> GSQPEQKTLSLPGTYRHVDRTTGQVLTCDKCPAGTYVSEHCTNMSLRVCSSCPAGTFTRHENGIERCHDCSQPCPWPMIERLPCAALTDRECICPPGMYQSNGTCAPHTVCPVGWGVRKKGTENEDVRCKQCARGTFSDVPSSVMKCKAHTDCLGQNLEVVKPGTKETDNVCGMRLFFSSTASGRGLVPR;> GSSTPDAVDKYLETPGDENEHAHFQKAKERLEAKHRERMSQVMREWEEAERQAKNLPKADKKAVIQHFQEKVESLEQEAANERQQLVETHMARVEAMLNDRRRLALENYITALQAVPPRPHHVFNMLKKYVRAEQKDRQHTLKHFEHVRMVDPKKAAQIRSQVMTHLRVIYERMNQSLSL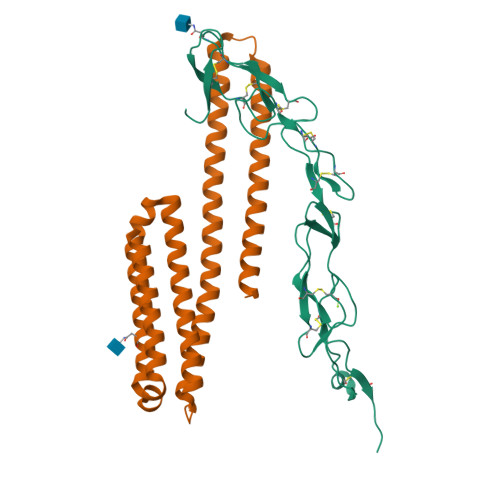LYNVPAVAEEIQDEVDELLQKEQNYSDDVLANMISEPRISYGNDASGRGLVPR(6~{S})-6-[2,4-bis(fluoranyl)phenyl]-~{N},~{N},4-trimethyl-2-oxidanylidene-5,6-dihydro-1~{H}-pyrimidine-5-carboxamide | 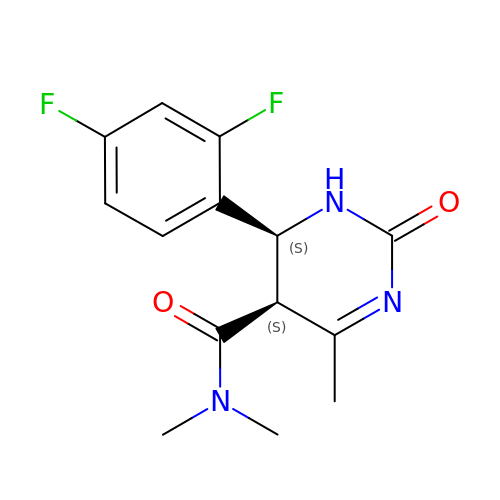C14 H15 F2 N3 O2 | MEHFDOJZBVYYGY-VXGBXAGGSA-N>GFEEALELTIRAKEEGDPRLLERALEILERRLKEAQERGDLHLVLTIALLLAAIAHRLGDPRYLEVAVRVLEEAIREALERGDVQLVYNLVEVLLHVARLLGDPRVFRFMLHILLEA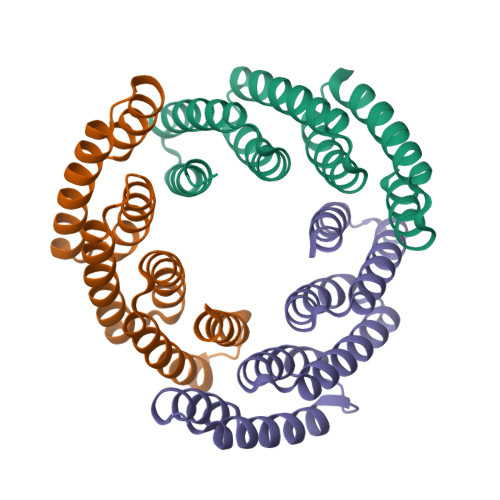YRIARENGDEQILIEIVHLFTEVIRG[3x]>MASMTGGQQMGRGSEFAKAPEQTVTEPVGSYARAERPQDFEGFVWRLDNDGKEALPRNFRTSADALRAPEKKFHLDAAYVPSREGMDALHISGSSAFTPAQLKNVAAKLREKTAGPIYDVDLRQESHGYLDGIPVSWYGERDWANLGKSQHEALADERHRLHAALHKTVYIAPLGKHKLPEGGEVRRVQKVQTEQEVAEAAGMRYFRIAATDHVWPTPENIDRFLAFYRTLPQD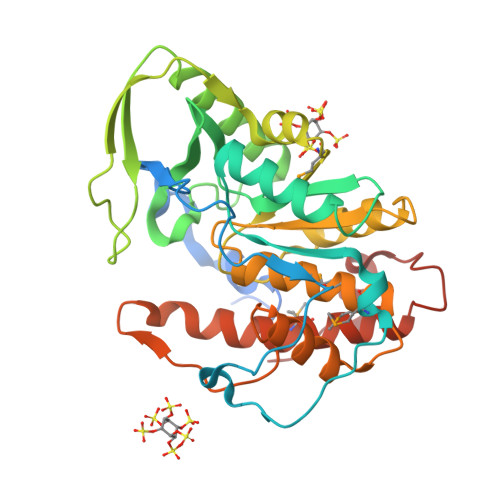AWLHFHCEAGVGRTTAFMVMTDMLKNPSVSLKDILYRQHEIGGFYYGEFPIKTKDKDSWKTKYYREKIVMIEQFYRYVQENRADGYQTPWSVWLKSHPAKALE[3x]{1-[(3-HYDROXY-METHYL-5-PHOSPHONOOXY-METHYL-PYRIDIN-4-YLMETHYL)-AMINO]-ETHYL}-PHOSPHONIC ACID | C10 H18 N2 O8 P2 | 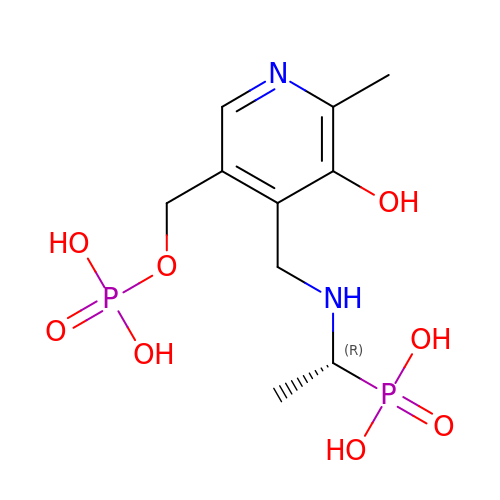WHDCJKAOZPBUAY-SSDOTTSWSA-N>[2x]MAYRKPSDLDGFIQQMPKADMRVKVQLAEDLVTFLSDDTNSIVCTDMGFLIDGLMPWLTGSHFKIAQKSLEAFSELIKRLGSDFNAYTATV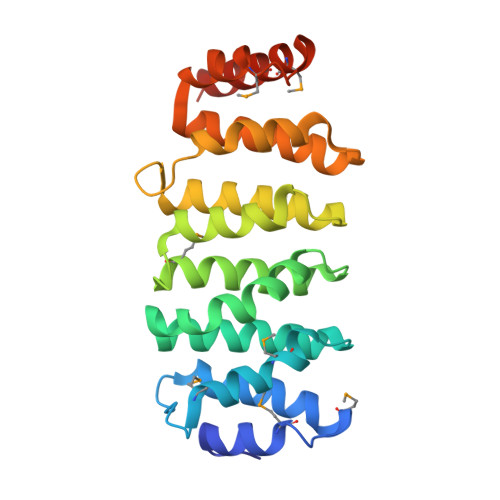LPHVIDRLGDSRDTVREKAQLLLRDLMEHRVLPPQALIDKLATSCFKHKNAKVREEFLQTIVNALHEYGTQQLSVRVYIPPVCALLGDPTVNVREAAIQTLVEIYKHVGDRLRPDLRRMDDVPASKLAMLEQKFDQVKLEHHHHHH> VAPGIVIPPKALFTQQGGAYGRCPNGT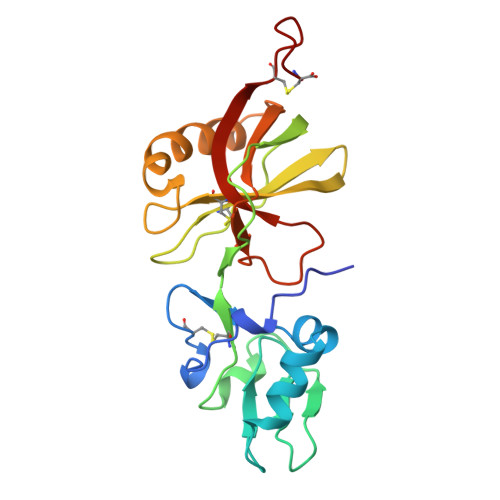RALTVAELRGNAELQTYLRQITPGWSIYGLYDGTYLGQAYGGIIKDAPPGAGFIYRETFCITTIYKTGQPAADHYYSKVTATRLLASTNSRLCAVFVRDGQSVIGACASPYEGRYRDMYDALRRLLYMIYMSGLAVRVHVSKEEQYYDYEDATFQTYALTGISLCNPAASIC PCNA encircling duplex DNA is quite stable and is removed from DNA by the dedicated clamp unloader Elg1-RFC. The three alternative RFC-like complexes are formed by replacement of the large subunit, Rfc1 of RFC, with Rad24, Ctf18, or Elg1 (16). Specifically, Elg1 contains two external loops that block opening of the Elg1-RFC complex for DNA binding, and an “Elg1 plug” domain that fills the central DNA binding chamber, thereby reinforcing the exclusive PCNA unloading activity of Elg1-RFC. In all three Elg1-RFC structures, we found five bound nucleotides: four ATPγS in Rfc2, Rfc3, Rfc4, and Elg1, and one ADP in Rfc5 (top right).

By leveraging state-of-the-art cryo–electron microscopy (cryo-EM), we find that the architecture of Elg1-RFC is specifically suited to the unloading of PCNA. This report documents Elg1-RFC alone and Elg1-RFC bound to a closed PCNA clamp and to a cracked PCNA clamp at 3.2-, 3.3-, and 3.7-Å resolution, respectively. Because clamp unloading starts with PCNA encircling dsDNA, we propose that the three structures that we have determined represent (i) Elg1-RFC alone before it encounters a PCNA, (ii) Elg1-RFC that has taken the PCNA off DNA with the clamp being incompletely closed (i.e., cracked PCNA), and (iii) Elg1-RFC bound to the closed PCNA after PCNA is taken off DNA (Elg1-RFC–closed PCNA), respectively. The shared Elg1-RFC among the three structures is highly similar with a root mean square deviation between main chain Cα atoms in the range of 0.5 to 0.6 Å. In the cracked PCNA ring, PCNA protomers 2 and 3 are slightly uplifted toward the unloader, disrupting the β sheet interface between a PCNA interface. Clamp loader disruption of a PCNA interface is also observed in the RFC-CNA-DNA complexes, but, in those cases, the PCNA forms a wide-open ring, guided by the large RFC conformational changes, and is a presumed intermediate in clamp loading rather than unloading. Once the interface of PCNA is cracked, it likely dissociates from DNA (right). It is also possible that the Elg1-RFC AAA+ domains may interact more fully with a transient destabilized form of PCNA, leading to the cracked ring structure observed herein. Thus, after binding of Elg1-RFC to PCNA and PCNA ring cracking, the PCNA ring can only be unloaded from DNA and not loaded onto DNA.

> MKRHVSLSDILTGNKRKVRRQDALQITIDDENDTESGTFDARTAKHDDSSVIFLNHSVVKPIEAVSTNHKSAKEFLMTKRTKEKCDDDDDDLIVISDKSPKSETNCSKIALSQEHEDDISIISTSRIKSSLLNERASKIKNFLKHETTDTFKRLNSISKLNEIEPPLPLHQSIFPVGDKELSDRSVDIPLPFRTIPPLNHNFLPSDYESLKDKNSASCIPVRYQAPVLLGTNIKRNTTLTWPQLFKPVTLKQVLIEPKLKLRIKNWIETSFHTLEKPTLRNRLLNRINPNKQQGSGDELANFIVPDLEEDENLRPDFYRNGEANSSLSEFVPLMILHGNSIGKKTLIQTIMREIAGDDNSYQIYEVNSNMNRSKKDLLDILLDFTTTHYVKDSSKRKSDYGLVLFNDVDVLFKEHDRGYWAMISKLCEFSRRPLVLTCKDLSLVPSELIALASEQNSLFHTKKISTSTVYAFLTKYLKSLEIEVCDDWLRDVVKQNNADIRKCLMHLQFWCVDTEADLISSKNRLPVLTSTLGSSVKDISQLTDLLSINDVIGQATLNRSMVRQEIDSTTMTPEKVNTFQDQNLDDEMKLKFDYVIDYKLHLNDPNRQPLLPFELNIYQHIQEQLEARYSYVREANHRLDNEYLVNRFKKMTESTLNFLASRIPKYDHLQSARRTRNSKKISDILNQFKGIYNDETLNENAEIDLLSATTQQIKAEINPFVFEIAKSDANVKNENKQIFELHSENVSERRYKDLVYQLSQEGVLKNVWFNADPSIVVRKWEHLHSGFSKNK;> MSKTLSLQLPWVEKYRPQVLSDIVGNKETIDRLQQIAKDGNMPHMIISGMPGIGKTTSVHCLAHELLGRSYADGVLELNASDDRGIDVVRNQIKHFAQKKLHLPPGKHKIVILDEADSMTAGAQQALRRTMELYSNSTRFAFACNQSNKIIEPLQSRCAILRYSKLSDEDVLKRLLQIIKLEDVKYTNDGLEAIIFTAEGDMRQAINNLQSTVAGHGLVNADNVFKIVDSPHPLIVKKMLLASNLEDSIQILRTDLWKKGYSSIDIVTTSFRVTKNLAQVKESVRLEMIKEIGLTHMRILEGVGTYLQLASMLAKIHKLNNKA;> MSTSTEKRSKENLPWVEKYRPETLDEVYGQNEVITTVRKFVDEGKLPHLLFYGPPGTGKTSTIVALAREIYGKNYSNMVLELNASDDRGIDVVRNQIKDFASTRQIFSKGFKLIILDEADAMTNAAQNALRRVIERYTKNTRFCVLANYAHKLTPALLSRCTRFRFQPLPQEAIERRIANVLVHEKLKLSPNAEKALIELSNGDMRRVLNVLQSCKATLDNPDEDEISDDVIYECCGAPRPSDLKAVLKSILEDDWGTAHYTLNKVRSAKGLALIDLIEGIVKILEDYELQNEETRVHLLTKLADIEYSISKGGNDQIQGSAVIGAIKASFENETV;> MFEGFGPNKKRKISKLAAEQSLAQQPWVEKYRPKNLDEVTAQDHAVTVLKKTLKSANLPHMLFYGPPGTGKTSTILALTKELYGPDLMKSRILELNASDERGISIVREKVKNFARLTVSKPSKHDLENYPCPPYKIIILDEADSMTADAQSALRRTMETYSGVTRFCLICNYVTRIIDPLASRCSKFRFKALDASNAIDRLRFISEQENVKCDDGVLERILDISAGDLRRGITLLQSASKGAQYLGDGKNITSTQVEELAGVVPHDILIEIVEKVKSGDFDEIKKYVNTFMKSGWSAASVVNQLHEYYITNDNFDTNFKNQISWLLFTTDSRLNNGTNEHIQLLNLLVKISQL;> MSLWVDKYRPKSLNALSHNEELTNFLKSLSDQPRDLPHLLLYGPNGTGKKTRCMALLESIFGPGVYRLKIDVRQFVTASNRKLELNVVSSPYHLEITPSDMGNNDRIVIQELLKEVAQMEQVDFQDSKDGLAHRYKCVIINEANSLTKDAQAALRRTMEKYSKNIRLIMVCDSMSPIIAPIKSRCLLIRCPAPSDSEISTILSDVVTNERIQLETKDILKRIAQASNGNLRVSLLMLESMALNNELALKSSSPIIKPDWIIVIHKLTRKIVKERSVNSLIECRAVLYDLLAHCIPANIILKELTFSLLDVETLNTTNKSSIIEYSSVFDERLSLGNKAIFHLEGFIAKVMCCLD;>[3x]ASMLEAKFEEASLFKRIIDGFKDCVQLVNFQCKEDGIIAQAVDDSRVLLVSLEIGVEAFQEYRCDHPVTLGMDLTSLSKILRCGNNTDTLTLIADNTPDSIILLFEDTKKDRIAEYSLKLMDIDADFLKIEELQYDSTLSLPSSEFSKIVRDLSQLSDSINIMITKETIKFVADGDIGSGSVIIKPFVDMEHPETSIKLEMDQPVDLTFGAKYLLDIIKGSSLSDRVGIRLSSEAPALFQFDLKSGFLQFFLAPKFNDEE> XSAVKAARYGKDNVRVYKVHKDEKTGVQTVYEMTVCVLLEGEIETSYTKADNSVIVATDSIKNTIYITAKQNPVTPPELFGSILGTHFIEKYNHIHAAHVNIVCHRWTRMDIDGKPHPHSFIRDSEEKRNVQVDVVEGKGIDIKSSLSGLTVLKSTNSQ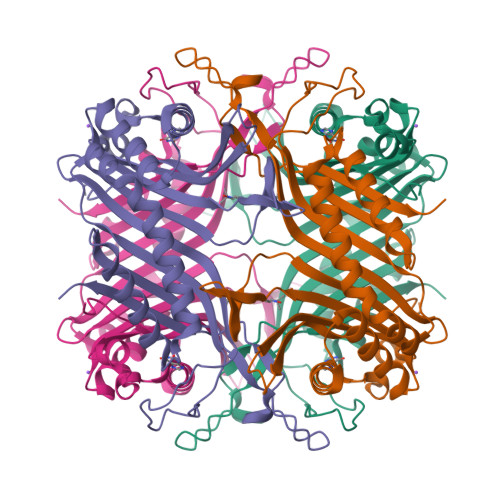FWGFLRDEYTTLKETWDRILSTDVDATWQWKNFSGLQEVRSHVPKFDATWATAREVTLKTFAEDNSASVQATMYKMAEQILARQQLIETVEYSLPNKHYFEIDLSWHKGLQNTGKNAEVFAPQSDPNGLIKCTVGRS> RAKVAMSHFEPHEYIRYDLLEKNIDIVRKRLNRPLTLSEKIVYGHLDDPANQEIERGKTYLRLRPDRVAMQDATAQMAMLQFISSGLPKVAVPSTIHCDHLIEAQLGGEKDLRRAKDINQEVYNFLATAGAKYGVGFWRPGSGIIHQIILENYAYPGVLLIGTDSHTPNGGGLGGICIGVGGADAVDVMAGIPWELKCPKVIGVKLTGSLSGWTSPKDVILKVAGILTVKGGTGAIVEYHGPGVDSISCTGMATICNMGAEIGATTSVFPYNHRMKKYLSKTGRADIANLADEFKDHLVPDPGCHYDQVIEINLSELKPHINGPFTPDLAHPVAEVGSVAEKEGWPLDIRVGLIGSCTNSSYEDMGRSAAVAKQALAHGLKC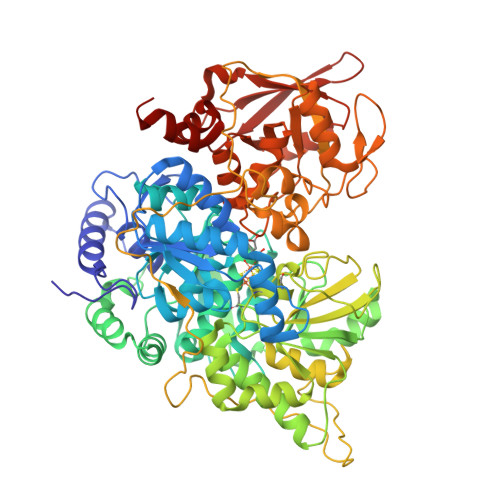KSQFTITPGSEQIRATIERDGYAQVLRDVGGIVLANACGPCIGQWDRKDIKKGEKNTIVTSYNRNFTGRNDANPETHAFVTSPEIVTALAIAGTLKFNPETDFLTGKDGKKFKLEAPDADELPRAEFDPGQDTYQHPPKDSSGQRVAVSPTSQRLQLLEPFDKWDGKDLEDLQILIKVKGKCTTDHISAAGPWLKFRGHLDNISNNLLIGAINIENRKANSVRNAVTQEFGPVPDTARYYKQHGIRWVVIGDENYGEGASREHSALEPRHLGGRAIITKSFARIHETNLKKQGLLPLTFADPADYNKIHPVDKLTIQGLKDFAPGKPLKCIIKHPNGTQETILLNHTFNETQIEWFRAGSALNRMKELQQK6-[2,6-bis(chloranyl)phenoxy]pyridin-3-amine | C11 H8 Cl2 N2 O | 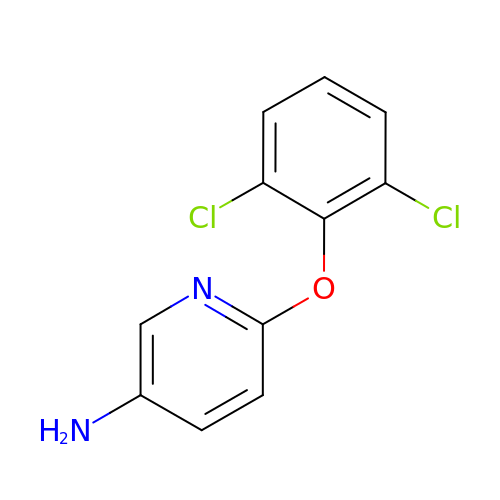YNVFZWPRJYWBOP-UHFFFAOYSA-N> MAGLASLSSVGALRGMRLVPAAHLLPLHSAFGQQTRNFGAGDLKIVAARMKSVKSIQKITKAMKMVAASKLRMDQRRLENGLPFATPVQKLVQRIPVDPKEKGTLAVLALSSDKGLCGGVNSFVAKQARIVIKENEMAGNAVQVYGVGDKIRSALQRTFGDRFKRIMTEVTRFPWNFGQACIIADRLMQDNPARLMVIYNHFKSAVAYDTLTLNVLTPTQAAQSAKEQLNTFEFEPEKTD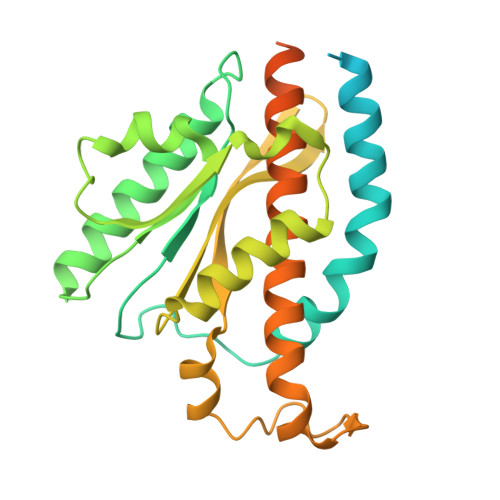VWKDLQDFYYACTVFGCMLDNIASEQSARMSAMDNASTNAGEMISSLTLRYNRARQAKITTELVEIISGANALE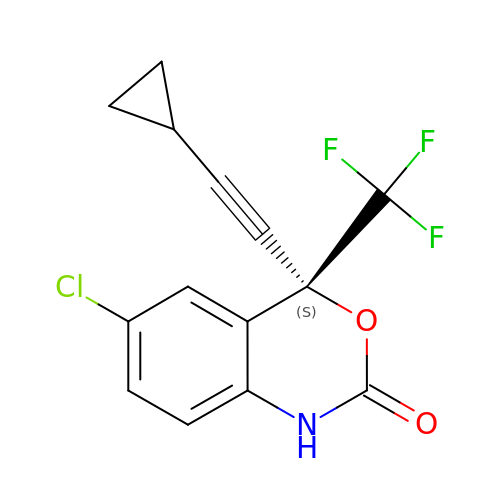(-)-6-CHLORO-4-CYCLOPROPYLETHYNYL-4-TRIFLUOROMETHYL-1,4-DIHYDRO-2H-3,1-BENZOXAZIN-2-ONE | C14 H9 Cl F3 N O2 | XPOQHMRABVBWPR-ZDUSSCGKSA-N> MTNIQTQLDNLRK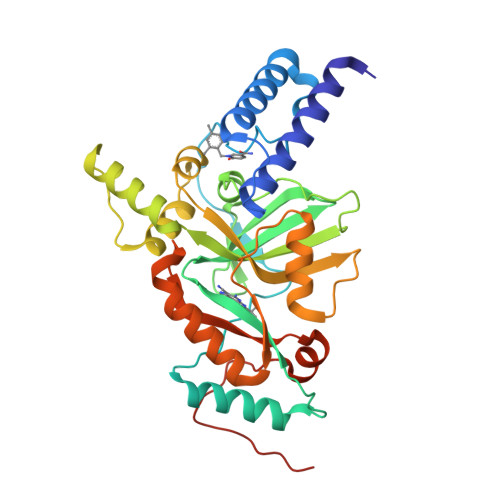TLRQYEYEYHVLDNPSVPDSEYDRLFHQLKALELEHPEFLTSDSPTQRVGAKPLSGFSQIRHEIPMLSLDNAFSDAEFNAFVKRIEDRLILLPKPLTFCCEPKLDGLAVSILYVNGELTQAATRGDGTTGEDITANIRTIRNVPLQLLTDNPPARLEVRGEVFMPHAGFERLNKYALEHNEKTFANPRNAAAGSLRQLDPNITSKRPLVLNAYGIGIAEGVDLPTTHYARLQWLKSIGIPVNPEIRLCNGADEVLGFYRDIQNKRSSLGYDIDGTVLKINDIALQNELGFISKAPRWAIAYKFPAQEELTL>[2x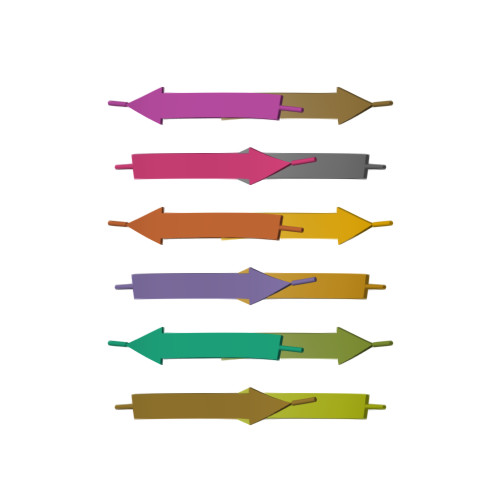]KLVFFA pentyl 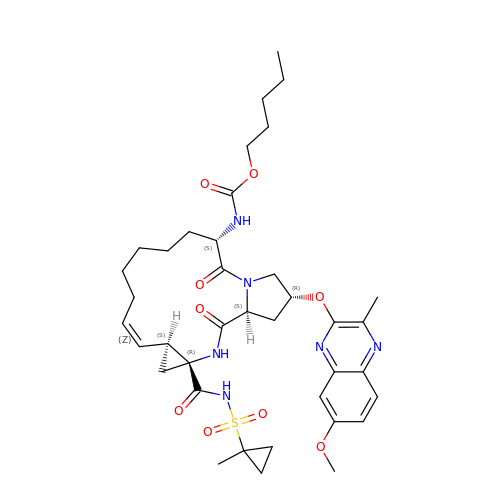[(2R,6S,12Z,13aS,14aR,16aS)-2-[(7-methoxy-3-methylquinoxalin-2-yl)oxy]-14a-{[(1-methylcyclopropyl)sulfonyl]carbamoyl}-5,16-dioxo-1,2,3,5,6,7,8,9,10,11,13a,14,14a,15,16,16a-hexadecahydrocyclopropa[e]pyrrolo[1,2-a][1,4]diazacyclopentadecin-6-yl]carbamate | C38 H52 N6 O9 S | XMVGSOUFSMLCKC-OJHKTYPMSA-N> GPLGSKSFTC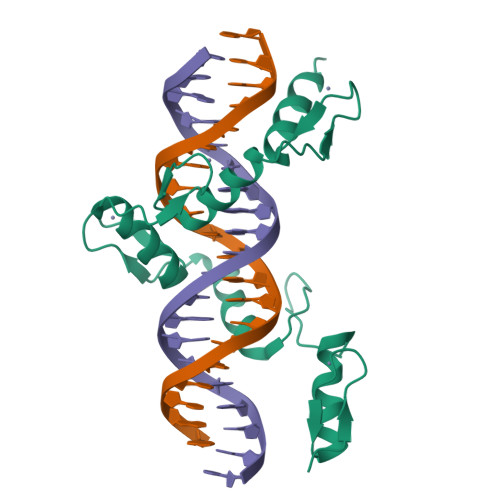DQCGKYFSQKRQLKSHYRVHTGHSLPECSHCHRKFMDVSQLKKHLRTHTGEKPFTCEICGKSFTAKSSLQTHIRIHRGEKPYSCSICGKCFSDSSAKRRHCILHTGKKPFSCPECGLQFARLDNLKAHLKIHSKEKHTADY> PGLSCRFYQHKFPEVEDVVMVNVRSIAEMGAYVSLLEYNNIEGMILLSELSRRRIRSINKLIRIGRNECVVVIRVDKEKGYIDLSKRRVSPEEAIKCEDKFTKSKTVY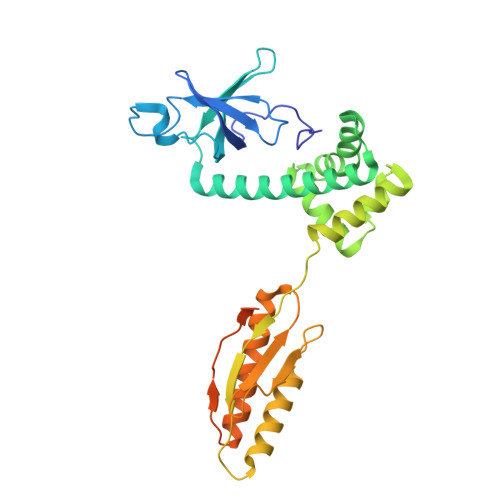SILRHVAEVLEYTKDEQLESLFQRTAWVFDDKYKRPGYGAYDAFKHAVSDPSILDSLDLNEDEREVLINNINRRLTPQAVKIRADIEVACYGYEGIDAVKEALRAGLNCSTENMPIKINLIAPPRYVMTTTTLERTEGLSVLSQAMAVIKEKIEEKRGVFNVQMEPKVVTDTDETELARQMERLERENAEVDGDDDAEEMEAKAED In contrast to the majority of carbapenemases, OXA-48-like carbapenemases have low activity toward carbapenems and show no significant hydrolysis of extended-spectrum cephalosporins, including CAZ. Here, we report the occurrence of single (OXA-48:P68A) and double (OXA-48:P68A,Y211S) amino acid substitutions within OXA-48 as a response to CAZ and CAZ-AVI exposure, respectively. The antimicrobial susceptibility data and enzyme kinetics showed that the P68A substitution was responsible for an increased activity toward CAZ, whereas P68A,Y211S led to a decrease in the inhibitory activity of AVI. X-ray crystallography structures revealed that OXA-48:P68A leads to increased flexibility within the OXA-48 structure, likely contributing to elevated CAZ hydrolysis.

In the first OXA-48:P68A structure (resolved to 2.50 Å), we found CAZ bound to chain A/C (OXA-48:P68A-CAZ), as well as two empty active sites (chain B/D, OXA-48:P68A)—thus, one CAZ molecule per dimer. In chains A and C of OXA-48:P68A-CAZ, CAZ was found covalently bound to the active-site residue S70 and stabilized by H-bonds involving residues S70, T209, Y211, S212, T213, R214, and R250. Comparing the CAZ unbound and bound chains of OXA-48:P68A, several conformational changes were evident. CAZ binding forces R214 in the β5-β6 loop to move out of the active site. As a result, R214 would then clash with parts of the Ω-loop (D143 to S165) in the native OXA-48. Indeed, we found residues 149 to 161 (for both chains A and C) in the Ω-loop of OXA-48:P68A to be disordered and thus not visible in the electron density maps. Therefore, P68A seems to impose increased flexibility within OXA-48, and this enables both the β5-β6 loop and Ω-loop to occupy alternative conformations and consequently favors CAZ binding. The X-ray structure of OXA-48:P68A with four chains in the asymmetric unit revealed that CAZ binding requires higher structural flexibility. In contrast, a strongly shortened β5-β6 loop and the absence of R214, as observed in OXA-163, expand the active-site cavity and allow OXA-163 to hydrolyze CAZ more efficiently. This supports the hypothesis that P68A increases the flexibility and changes the plasticity of the substrate binding site in OXA-48, allowing the hydrolysis of bulkier drugs such as CAZ. While OXA-48:P68A allows CAZ binding by a displacement of the β5-β6 and Ω-loops, we hypothesize that for other cephalosporins, the active site of OXA-48:P68A might still be too narrow and rigid to achieve significant hydrolysis.

>MRVLALSAVFLVASIIGMPAVAKEWQENKSWNAHFTEHKSQGVVVLWNENKQQGFTNNLKRANQAFLAASTFKIPNSLIALDLGVVKDEHQVFKWDGQTRDIATWNRDHNLITAMKYSVVPVYQEFARQIGEARMSKMLHAFDYGNEDISGNVDSFWLDGGIRISATEQISFLRKLYHNKLHVSERSQRIVKQAMLTEANGDYIIRAKTGYSTRIEPKIGWWVGWVELDDNVWFFAMNMDMPTSDGLGLRQAITKEVLKQEKIIP[4x]> AAPKAPADGL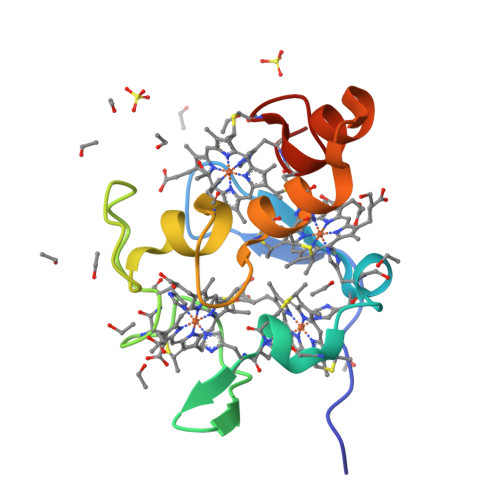KMDKTKQPVVFNHSTHKAVKCGDCHHPVNGKEDLQKCATAGCHDNMDKKDKSAKGYYHAMHDKGTKFKSCVGCHLETAGADAAKKKELTGCKGSKCHS> GAEKEDLVQEGILGLLKAIKFYDETKSSFSSFAFLCIRREMISAIRKANTQKHMVLNEALKTNAILEDSAYFDDEGHNINNY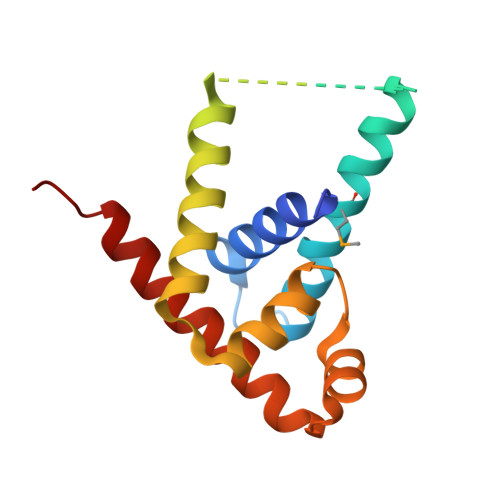KSSESNPEEAYLLKEEIEEFKKFSENNFSKFEKEVLTYLIRGYSYREIATILSKNLKSIDNTIQRIRKKSEEWIKEEENIKR2-amino-N-[(1S)-1-{8-[(1-methyl-1H-pyrazol-4-yl)ethynyl]-1-oxo-2-phenyl-1,2-dihydroisoquinolin-3-yl}ethyl]pyrazolo[1,5-a]pyrimidine-3-carboxamide | C30 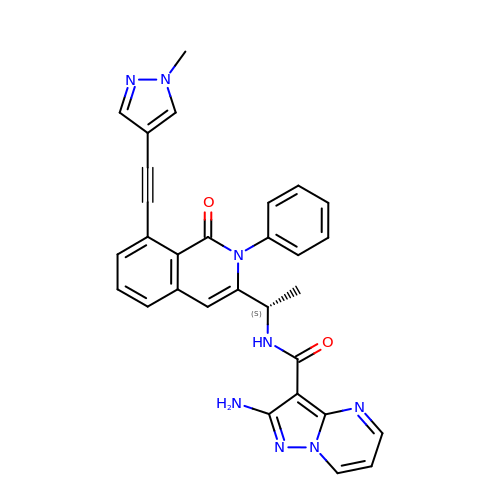H24 N8 O2 | XUMALORDVCFWKV-IBGZPJMESA-N N-(2-{[4-(hydroxyamino)-4-oxobutyl](methyl)amino}ethyl)benzamide 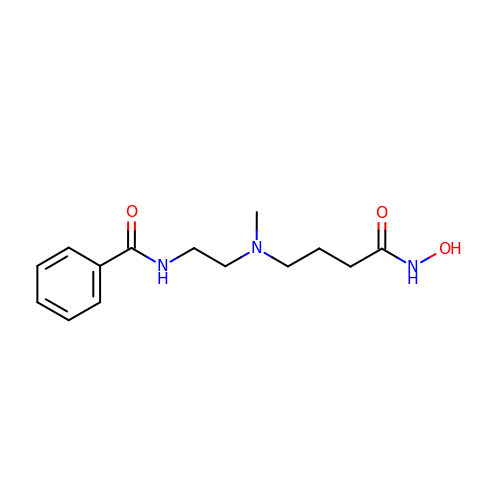| C14 H21 N3 O3 | WOJAVXMANLPPBT-UHFFFAOYSA-N> FKIYAKNYFLTYPNCSLSKEEALSQLKNLETPTNKKYIKVCRELHENGEPHLHVLIQFEGKYQCKNQRFFDLVSPNRSAHFHPNIQAAKSSTDVKTFVEKDGDFIDF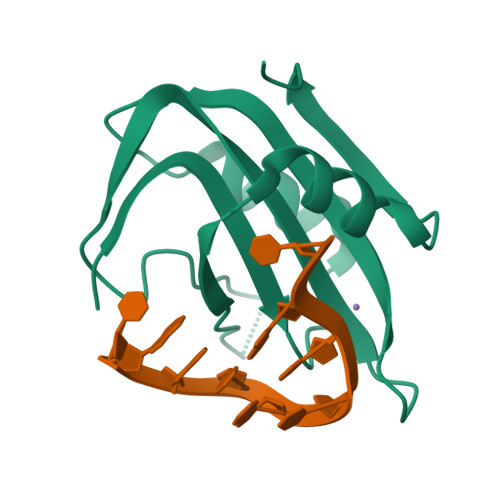GVFQI>MSNGILSQSIANMQQAEATIQSFSGLPQNAVNIQQNVGEVVAALLPQVQTMQQQVLAFAARLELQLTQQLANTGPFNPEALKAFVDLVQQEIAPIQTLTAQTLTASQSANDRITQDNIALQRIGVELQATIAGLQSNLDGARQELDSLNKKKLYLT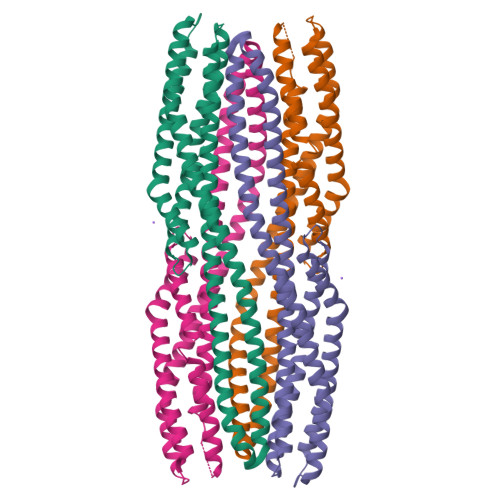GLGTTGLPGLIALAVTLTQTQNKVSSLEGQVNQIEGQIQRQQGFLGQTTAFSQQFGSLIDRVSKVGNTISLLGGDIANVARDAGQGDPELARLFFTAALTEVRTLQVDASHHHHHH[2x]>[3x]PPGPPGPPGFRGPA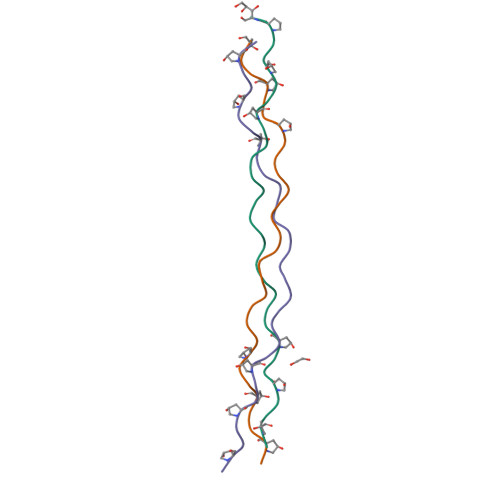GPNGIPGPPGPPGPPG>[2x]IKCPQPKTLDEFTIIQNLQPQYQFRDYFIATCKQGYQLIEGNQVLHSFTAVCQDDGTWHRAMPRCKIKDCGQPRNLPNGDFRYTTTMGVNTYKARIQYYCHEPYYKMQTRAGSRESEQGVYTCTAQGIWKNEQKGEKIPRCLPVCGKPVNPVEQRQQIIGGQKAKMGNFPWQVFTNIHGRGGGALLGDRWILTAAHTLYPKEHEAQSNASLDVFLGHTNVEELMKLGNHPIRRVSVHPDYRQDE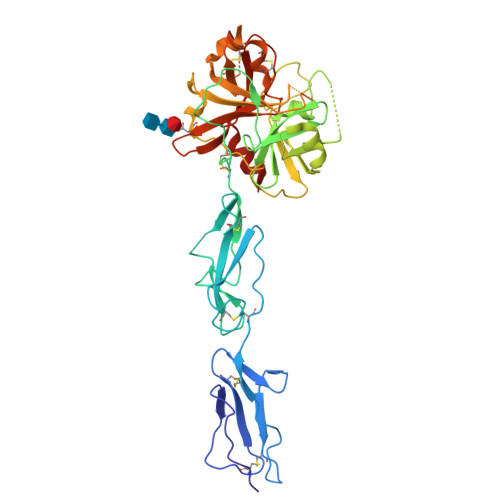SYNFEGDIALLELENSVTLGPNLLPICLPDNDTFYDLGLMGYVSGFGVMEEKIAHDLRFVRLPVANPQACENWLRGKNRMDVFSQNMFCAGHPSLKQDACQGDSGGVFAVRDPNTDRWVATGIVSWGIGCSRGYGFYTKVLNYVDWIKKEMEEED>[2x]ASAWPEEKNYHQPAILNSSALWQIAEGTSISEMWQNDLQPLLIERYPGSPGSYAARQHIMQRIQRLQADWVLEIDTFLSQTPYGYRSFSNIISTLNPTAKRHLVLACHYDSKYFSHWNNRVFVGATDSAVPCAMMLELARALDKKLLSLKTVSDSKPDLSLQLIFFDGEEAFLHWSPQDSLYGSRHLAAKMASTPHPPGARGTSQLHGMDLLVLLDLIGAPNPTFPN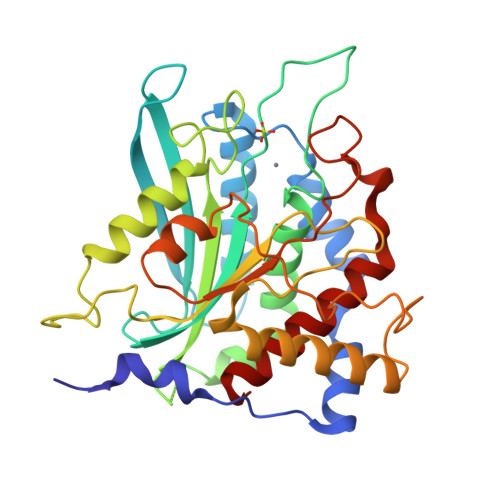FFPNSARWFERLQAIEHELHELGLLKDHSLEGRYFQNYSYGGVIQDDHIPFLRRGVPVLHLIPSPFPEVWHTMDDNEENLDESTIDNLNKILQVFVLEYLHL> GSHMEEMIRSL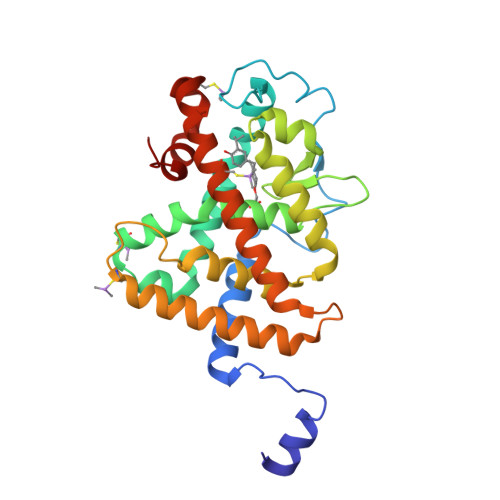QQRPEPTPEEWDLIHIATEAHRSTNAQGSHWKQRRKFLPDDIGQSPIVSMPDGDKVDLEAFSEFTKIITPAITRVVDFAKKLPMFSELPCEDQIILLKGCCMEIMSLRAAVRYDPESDTLTLSGEMAVKREQLKNGGLGVVSDAIFELGKSLSAFNLDDTEVALLQAVLLMSTDRSGLLCVDKIEKSQEAYLLAFEHYVNHRKHNIPHFWPKLLMKVTDLRMIGACHASRFLHMKVECPTELFPPLFLEVFEDQEV>MGSSHHHHHHSSGLVPGRGSMKLTIERAALLKALGHVQSVVERRNTIPILSNILLSAEGDRLSFSATDLDMEIIDEGFAQIDVPGQITAPAHTLYEIVRKLPDGADVSLSFSGDDPRLVIQAGRSRFNLPVLPAGDFPVMSSDGLSSRIAVDTNELIRLIDKTRFAISTEETRYYLNGLYVHTVNEGGETKLRAVATDGHRLALAEMPAPEGAVGIPGVIVPRKTIAEARRLMESAGETVDLQVSPQKVRFEFGAAALTSKVIDGAFPDYMRVIPRDNAKILTLDNDLFAKAVDRVATISAEKSRSVKLAVEPGRITLTVRNMEAGQAVEEVEVD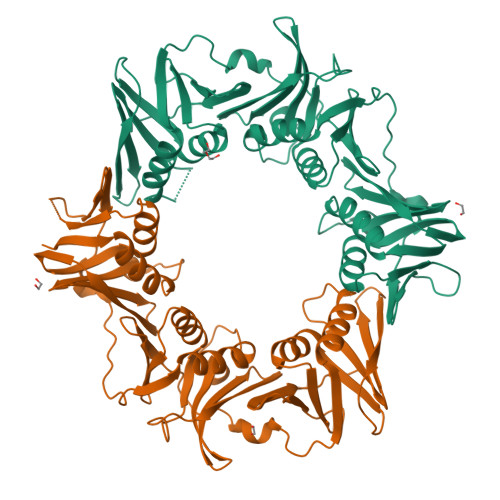YDGEPFEIGFNARYLLDVCGQIAGPQAEFRFADPASPTLVVDPVDPGVKYVLMPLRV[2x]>[2x]MGEELREEERGEVRSELITKGEKKLVLIRWNTGKTSAGRLFGRYGPGGRPEFFKLLFGAVAGSLREQFGPDGENIFNRIRDSEKFRETSRELFDGLK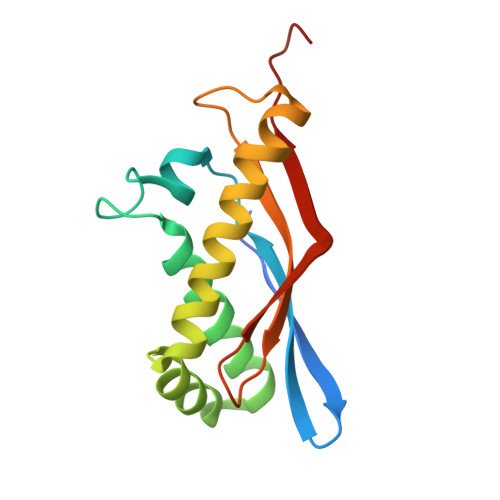KWFFEEAVPRYNLERGDIFMISTELVLDPDTGELLWNRDKTQLIYWIRSDR> GSINMATVPVYCVCRLPYDVTRFMIECDACKDWFHGSCVGVEEEEAPDIDIYHCPN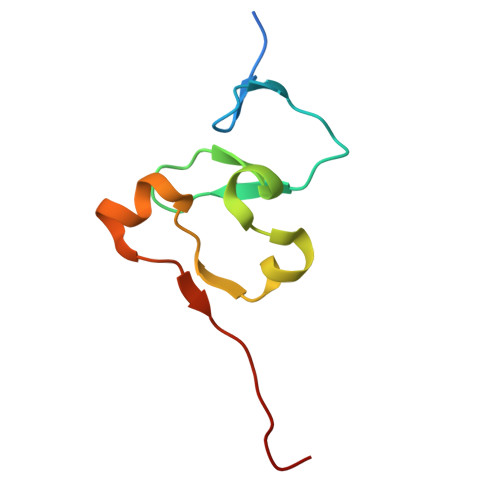CEKTHGKSTLKKKRTWHK> MEDFKKIVNNIRLKDTFDFKLAAFPNQNYDQLLPSQIYKNYYQGIEIQQHKYQNELDIKIINFLYPDGDFGSANKNGTLKLSLMLTDKKNNQVYYKLL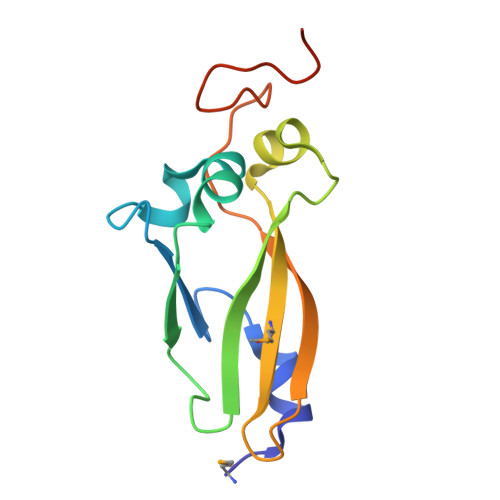EVSGFKSNPYGVDENGTIPGLEHHHHHH> MGHHHHHHMERVSITERPDWREKAHEYGFNFHTMYGEPYWCEDAYYKLTLAQVEKLEEVTAELHQMCLKVVEKVIASDELMTKFRIPKHTWSFVRQSWLTHQPSLYSRLDLAWDGTGEPKLLENNADTPTSLYEAAFFQWIWLEDQLNAGNLPEGSDQFNSL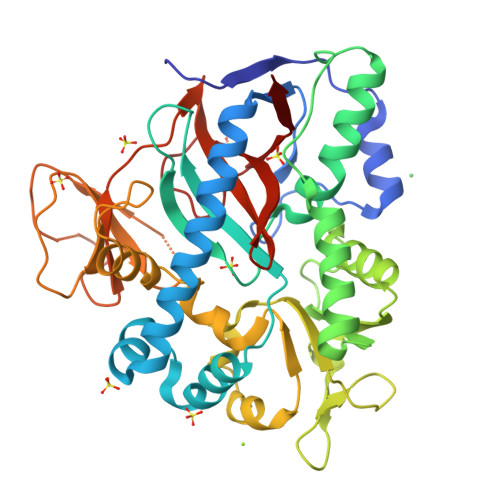QEKLIDRFVELREQYGFQLLHLTCCRDTVEDRGTIQYLQDCATEAEIATEFLYIDDIGLGEKGQFTDLQDQVISNLFKLYPWEFMLREMFSTKLEDAGVRWLEPAWKSIISNKALLPLLWEMFPNHPNLLPAYFAEDDHPQMEKYVVKPIFSREGANVSIIENGKTIEAAEGPYGEEGMIVQQFHPLPKFGDSYMLIGSWLVNDQPAGIGIREDRALITQDMSRFYPHIFVE cyclopentyl 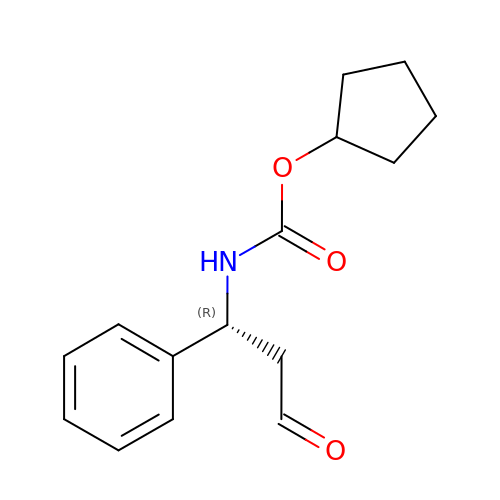N-[(1R)-3-oxidanylidene-1-phenyl-propyl]carbamate | C15 H19 N O3 | JHRUSYOIALPZLD-CQSZACIVSA-N> SFDASAYDAYIVQAVRGTMATNTENTMSLDDIIGMHDVKQV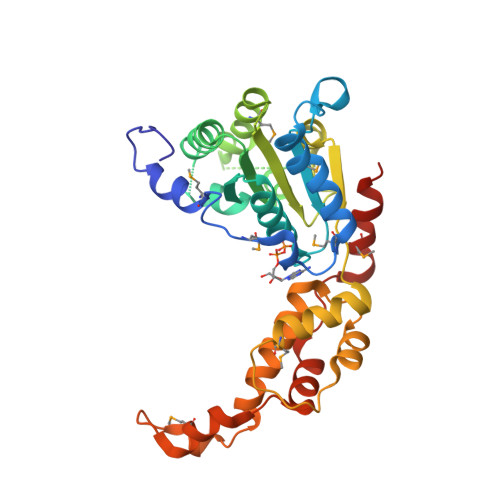LHEAVTLPLLVPEFFQGLRSPWKAMVLAGPPGTGKTLIARAIASESSSTFFTVSSTDLSSKWRGDSEKIVRLLFELARFYAPSIIFIDEIDTLGGQRGNSGEHEASRRVKSEFLVQMDGSQNKFDSRRVFVLAATNIPWELDEALRRRFEKRIFIPLPDIDARKKLIEKSMEGTPKSDEINYDDLAARTEGFSGADVVSLCRTAAINVLRRYDTKSLRGGELTAAMESLKAELVRNIDFEAALQAVSPSAGPDTMLKCKEWCDSFGAM>GPGSDVANAVDTEAPQVKTGDYVVYRGESFEFYAEITDNSGQVNDVVVRNVELDKKTSQPYLTPGFIKFSTDNLGLPGNATVQNPLRTKIFGTVPLNEGIGYYTRYVVPTDSNGNTTRMVQNDNRNGLERF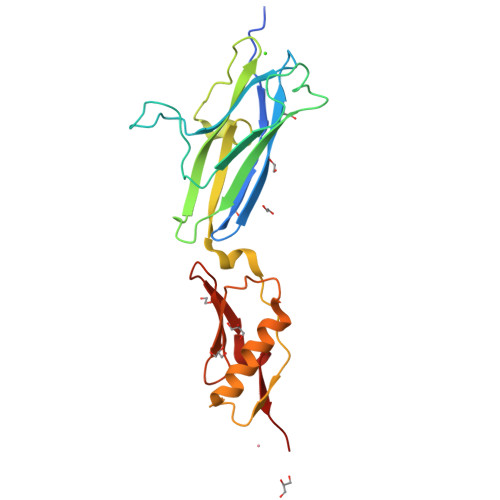IITIKTQNEKYNPADPAITYVNQLSNLSQAERDAVAAAVRTANPQIPAAARITVSANGTVTITYPDSSTDTIPADRVVKDLAS[2x]>SVKLAGNSSLCPVSGWAIYSKDNSVRIGSKGDVFVIREPFISCSPLECRTFFLTQGALLNDKHSNGTIKDRSPYRTLMSCPIGEVPSPYNSRFESVAWSASACHDGINWLTIGISGPDNGAVAVLKYNGIITDTIKSWRNNILRTQESECACVNGSCFTVMTDGPSNGQASYKIFRIEKGKIVKSVEMNAPNYHYEECSCYPDSSEITCVCRDNWHGSNRPWVSFNQNLEYQIGYICSGIFGDNPRPNDKTGSCGPVSSNGANGVKGFSFKYGNGVWIGRTKSISSRNGFEMIWDPNGWTGTDNNFSIKQDIVGINEWS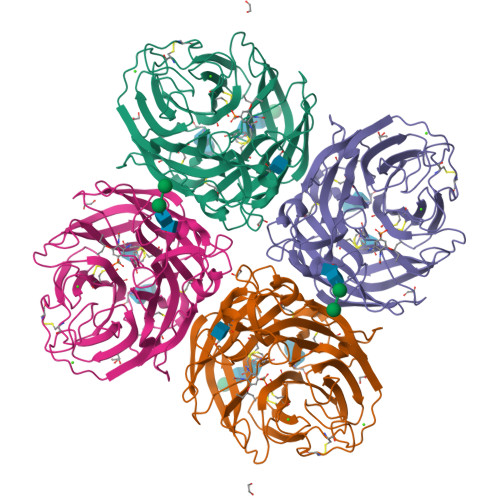GYSGSFVQHPELTGLDCIRPCFWVELIRGRPKENTIWTSGSSISFCGVNSDTVGWSWPDGAELPFTID[2x]>[2x]SMLAELITSYRKSAAIYAFVDTGLSIHFRNGAYVDIDELSRQCGIDYSRLDRLCDFLIEIGILVNHGHKVTLSEECSALADPESMESLIVKWELSPDCWNAWSMYPRSLL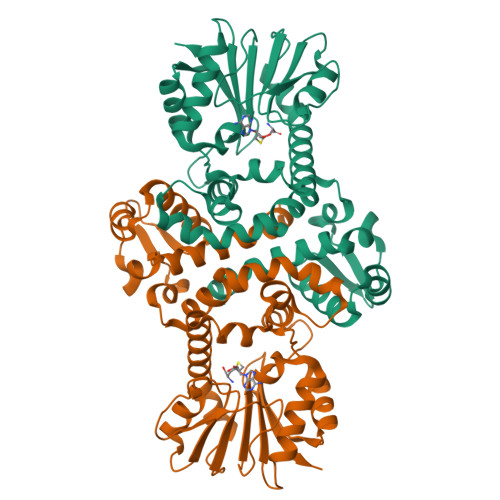ENDGKPAFEITHGKSFFEHLASNKLLKSNFDSSMSKGSDKIIEKLLDIYDFGQYNRILDIGGGEGSLLVKMSEKVKGKHYAVLDRYDEIPVLENIDFINGDFLKVIPSGYDLYILKDVIHDWSDNNAILILENCRKAMDNGSAVLLISYMKKPQSKMVIYLDILMDVLFSGKERYLTEFERLANQAGLVIQDVKDIDESSSIIQLGIK> ANELTWHDVLAEEKQQPHFLNTLQTVASERQSGVTIYPPQKDVFNAFRFTELGDVKVVILGQDP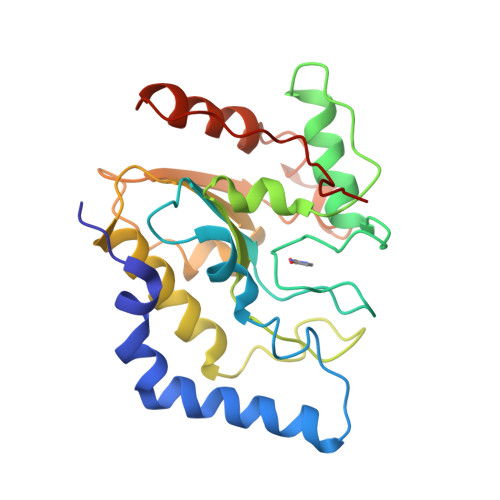YHGPGQAHGLAFSVRPGIAIPPSLLNMYKELENTIPGFTRPNHGYLESWARQGVLLLNTVLTVRAGQAHSHASLGWETFTDKVISLINQHREGVVFLLWGSHAQKKGAIIDKQRHHVLKAPHPSPLSAHRGFFGCNHFVLANQWLEQHGETPIDWMPVLPAESE(5R)-N-benzyl-5-ethyl-1-methyl-1,4-diazepane-5-carboxamide | 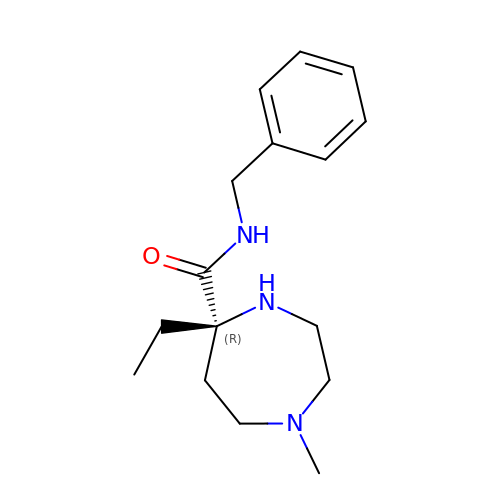C16 H25 N3 O | HCTANGJAFMIUKA-MRXNPFEDSA-N> MEEGGSTGSAGSDSSTSGSGGAQQRELERMAEVLVTGEQLRLRLHEEKVIKDRRHHLKTYPNCFVAKELIDWLIEHKEASDRETAIKLMQKLADRGIIHHVCDEHKEFKDVKLFYRFRKDDGTFPLDNEVKAFMRGQRLYEKLMSPENTLLQPREEEGVKYERTFMASEFLDWLVQEGEATTRKEAEQLCHRLMEHGI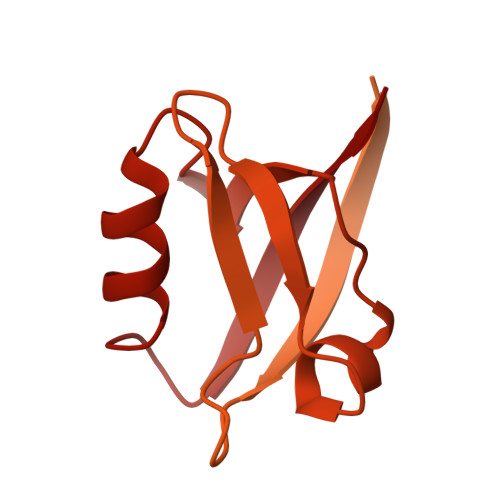IQHVSSKHPFVDSNLLYQFRMNFRRRRRLMELLNEKSPSSQETHDSPFCLRKQSHDNRKSTSFMSVSPSKEIKIVSAVRRSSMSSCGSSGYFSSSPTLSSSPPVLCNPKSVLKRPVTSEELLTPGAPYARKTFTIVGDAVGWGFVVRGSKPCHIQAVDPSGPAAAAGMKVCQFVVSVNGLNVLHVDYRTVNNLILTGPRTIVMEVMEELEC> YFGTLTQKAPNWYRCSSTRAKEEVVGH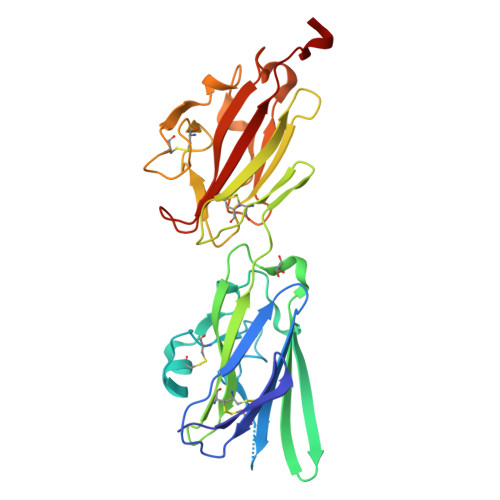VTLNKEHPDMTIECVDDGLGGEFLPLEGARSSYPRVCHIDAKDQDDCERNRGFLTDYIPGAKQYWYKIEKVEQNGEQSVLYKFTVPWILLPPAKQRYKVGCRYPNHEYCFVEVTVEPTPPMVEGKRVTCGYSESGPVNLEVDLSKNANFIEIRCGEQHHPQPSTYTLQYCSGDSVDPQKCSPQSLTNIFYDYSSSWWKGKLNGPDGATLTIPPGGFPEEDKSFLVGCSLTVDGPPFCNVKVRVAGNPAAALV> MNINVPDATRIGRATGAKAPEFQELYDFDAAALTLTSAVFPYDSQIHRAHVVMLTEQGILTVEESATILSGLAQVDELAATDGSLRTYL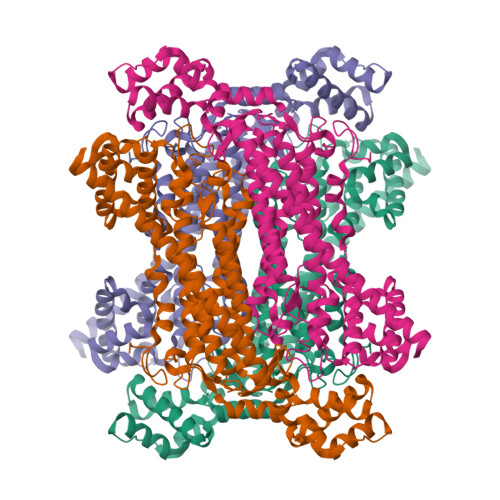PYEAALKRTIGSVAGKMHIGRSRNDLANAGKRMFLRDQLLRTIEAVIGYREAVVHKAADHLDTVMVVYTQRKEAQPITLGHYLMAISENLAKNLDRYRELYARINLCPLGAAATAGTGWPLNRDRTSALLGFDGLVVNSIEGVAGWDHVAEHAFVNAVFLSGLSRLASEIQLWSTDEYQVAELDASFAGTSSIMPQKKNPDSLERSRKAAFAAMGPLVGILTSLNAIEYQYSAARVELEPRSIDALIAATHAMTGVVRTLHPNKERMRQYAAENYSTMTDLTDMLVRRVGIDYREAHEIVAHVVITAIEKGIKANKIGLDLVQEAAVAQTGAGINVSADDIKDALDPWQNVLRREGKGMPAPMSVKASIDDAMAELHKDRAWLANATQALANAKQTLADSVQQIIQTDRKYLRHHHHHH Myophage Mu is a representative of contractile nanomachines with a simple tail baseplate. It has the capacity to infect a range of intestinal bacteria and has extensive applications in genetic engineering research. Using cryo-EM, we resolved the three-dimensional (3D) structures of the G(+) type phage Mu in both its extended state and urea-induced contracted state, the latter lacking the baseplate, at near-atomic resolutions. The structure of extended Mu can be divided into four distinct regions: the DNA-containing head, the connector complex, the tail, and the baseplate.

The baseplate was classified and reconstructed by using RELION software, generating a final resolution of 3.3 Å. The simple baseplate is comprised of eight protein components, including a hexameric tube initiator (gp43), a trimeric hub (gp44), a trimeric spike (gp45), six wedges (one BW1 gp46, two BW2 gp47, and one BW3 gp48), and six trimeric fibers (gp49 and gp50). The tube initiator protein gp43 is composed of two domains: a tube-like domain and a helix-rich domain, which are connected by a flexible loop. The tube-like domains from six copies of gp43 form a 24-stranded β-barrel hexamer, analogous to that of the tube gp40, which serves to initiate the assembly of the tail tube. It is noteworthy that the helix-rich domain comprises eight α-helixes, which extend downward and form extensive interactions with the baseplate wedges. The Mu spike protein gp45 is comprised of three domains: an oligosaccharide-binding (OB-fold) domain, a β-helical domain, and an apex domain, which may have the function of binding and penetrating the cell membrane. It is noteworthy that two additional spherical densities, which are presumed to be Fe and Ca ions, are present in the apex domain of the spike gp45, which is consistent with the reported X-ray crystal structure. As with myophages Milano, E217 (14), and Pam3 (13), the baseplate wedge of Mu is composed of six heterotetramers, each comprising one BW1 gp46, one BW3, and two conformers of BW2 (referred to as BW2-i and BW2-o). Moreover, the entire three-helical bundle is embedded between the helix-rich domains of two adjacent tube initiator gp43, thereby stabilizing the BWs into the baseplate. Based on our density map, we only built the atomic model for the N-terminus of protein gp49, which is anchored to the fiber docking loop (residues 133–155) of the BW3.

>[6x]MFEDALNAVNAVRDKTGGGRKTTGKGTFRNVPFLVIEEQKQAGGRRLVKREYPLRDTGGVNDLGKKLRSRTFSACILNSNAETARDEAGALMDALDAPGSGELVHPDFGTVDVMVDSWECRTKADELNYYAFTVTVYPSLQDTAPDAETDTSAAVPAQAVAVTGSLGDTLSSVWQTVKDGTAAATAVMEAVTGVIDDISDAVDNLGVTQTVSGLMGSLSAMKGSVTSLINQPAMLASSLMGALSGVSSLCDTRTAFSTWNRLAQRFERRHAATAGRQGTITTSYNSPVAEKNIATLNYVMLAAAQTYRAEAASQALTAALDFSRRMDNAARAPVLDAPSTTTGTASGASSTSATVTQGQLQLTAITPDGGFSQVSFSDSGTATPPVFESVSDIEKTTAMLGAALDSVILTASEQGFSTDSVQLTQLRLLVVADLEKRGLQLAGSESHHLPETLPAMVALYRFTGNSRNWQRLARRNGISNPLFVPGGVSIEVINE;>[6x]MSDISFNAIPSDVRVPLTYIEFDNSNAVSGTPAPRQRVLMFGQSGSKASAAPNVPVRIRSGSQASAAFGQGSMLALMADAFLNANRVAELWCIPQGNGTGNAAVGEISLSGTAGENGSLVTYIAGQRLAVSVAAGATGAALADLLVARIKGQPDLPVTAEVRADSGDDDTHADVVLSAKFTGALSAVDVRWNYYAGETTPYGIITAFKAASGKNGNPDISASIAGMGDLQYKYIVMPYTDEPNLNLLRTELQERWGPVNQADGFAVTVLSGTYGDISTFGVSRNDHLISCMGIAGAPEPSYLYAATLCAVASQALSIDPARPLQTLTLPGRMPPAVGDRFTWSERNALLFDGISTFNVNDGGEMQIERMITMYRTNKYGDSDPSYLNVNTIATLSYLRYSLRTRITQKFPNYKLASDGTRFATGQAVVTPSVIKTELLALFEEWENAGLVEDFDTFKEELYVARNKDDKDRLDVLCGPNLINQFRIFAAQVQFIL;>MAGNQRQGVAFIRVNGMELESMEGASFTPSGITREEVTGSRVYGWKGKPRAAKVECKIPGGGPIGLDEIIDWENITVEFQADTGETWMLANAWQADEPKNDGGEISLVLMAKQSKRIA[6x];>MTDLAIIWTNGRGDIAQDGIDMLTDDSLTTDVTISLFTDRRALDSDTLPDGSDDRRGWWGDSYRDRPIGSRLWLLSREKATPDTLERARGYAEEALEWLKTAGRVSAINVRAEQLHQGWLYLYIALTLPDGSVIPYEFKAAFNGV[6x];>MSNTVTLRADGRLFTGWTSVSVTRSIESVAGYFELGVNVPPGTDLSGLAPGKKFTLEIGGQIVCTGYIDSRRRQMTADSMKITVAGRDKTADLIDCAAVYSGGQWKNRTLEQIARDLCAPYGVTVRWELSDKESSAAFPGFTLDHSETVYEALVRASRARGVLMTSNAAGELVFSRAASTATDELVLGENLLTLDFEEDFRDRFSEYTVKGYARANGAEGDDIDAKSIVSRKGTATDSDVTRYRPMIIIADSKITAKDAQARALREQRRRLAKSITFEAEIDGWTRKDGQLWMPNLLVTIDASKYAIKTTELLVSKVTLILNDQDGLKTRVSLAPREGFLVPVESDRKNRKGGDSNGGIDALVEDYYRRHPEKTPPWKE[3x];>MAYSPPTLSSLIARTEQNIEQRLPGSWPQAREKTLSAIAYAQAGLAAGCHEHISWVGRQIIPSTADEDELLEHCRFWGVRRKQATAASGPLTVTTSAATTIPAGTRWQRADGVVYSLADTIVIDRAGTTEITVTALAAGEAGNTGENTLLTLITPVACVVSDAITVKGFSGGADIESAAELLSRLEYRVQYPPFGGNQFDYVRWAREVSGVTRAWCFPTWKGGGTVGVTFVMDNRSNIFPQPADVERVADYIAGHTDPITGLIVGQPDGVNVTVFAPKAKPVNPRIYISPKTAELKQAITNAINTMFFNEVMPGGALAPSRIIRAVAGVTGLDDFEVRFPTEIQRSENTELLTAGTIEWL[12x];>MERVNDSALNRLLTPLMRRVRLMLARAVVNVINDGRKVQNLQVGLLDDEESDEVERLQNYGHFSVPLPGAEALIACVGAQRDQGIAVVVEDRRYRPTNLEPGDAGIYHHEGHRIRLTKDGRCIITCKTVEVYADESMTVDTPRTTFTGDVEIQKGLGVKGKSQFDSNITAPDAIINGKSTDKHIHRGDSGGTTGPMQ[3x];>MAVTPWQTAFLQLLPSGLAWNKSPDSKLSALAQAISDVIATAADDARQMLRERFPSTSRWYLGEWESFLGLPDCTSENGTLSERQRAAANKMRMTGNLSRRFYEWLAAQYGFTVRLTDSTEGQWVTQVNIYGIKNYRNATVLDNVLTPLRVYESGALECLLEKYKPAHQIYKFVYHDGDN[6x];>[3x]MTGKRLKASVIIDLNGNLSRRSRQYSNQINALSRSGQSSLRALRMEVVRVSGAIDRMGSLSTRTFRMLSAGALGIAGVGYTANKLFIGAAAQREQQIIAMNSLYHGDKVRAQAMMAWAKQNAKDTTWGLSGVLDEIRSSKGFGMTDEQTKQFITMLQDQGAMHGWDLPTAQGASLQLKQMFARQQITAADANLLTGYGINVYQALADATGTDVKKIRDLGTKGKLGMKSILTVFRTLSEQSKGAQASAMNSWDGMFAQMEANLLEFRIKVANSGPFEEIKNEMRRVLNWHDMADKSGELDALAENIGQKFLTTFRTVKISAQELWRWLKPGKDALAWVDQNIVSLKKLAAVLVSVWLANKALRAGWAVAKPSWQVASYPFKTGRRMWRWMRNRKRGQAGLPVPDAMTSETLLQGIGIQRVFVINWPRGFGDYGSGGGRRVRSGGRMAPLLPRQPLLLSGPQPLALPAPRPVLALPPPGVPVTARPAPLPLPGKSGLLSRLAGSAAGQLVTGTVGKLADAGRAVGGWFSGIGNKLAGSAIGRVVTKGAGALGWMGKGAGRALSRLGGPVMGALQLAPVLMDEQASTHEKAGAIGSTAGAWLGGAVGSLAGPLGTVAGATLGSVAGEYLGGFVTDLYQKWTATDKEPQEQKVNAEASLRVELGEGLRLTSSRVTEDGMGLNIYAGDNYITGW;>[9x]MFYIDNDSGVTVMPPVSAQRSAIVRWFSEGDGNNVITWPGMDWFNIVQAELLNTLEEAGIQPDKTKLNQLALSIKAIMSNNALLIKNNLSEIKTAGASAQRTARENLDIYDASLNKKGLVQLTSATDSPSETLAATAKAVKIAMDNANARLAKDRNGADIPNKPLFIQNLGLQETVNRARNAVQKNGDTLSGGLTFENDSILAWIRNTDWAKIGFKNDADSDTDSYMWFETGDNGNEYFKWRSKQSTTTKDLMNLKWDALSVLVNAIVNGEVISKSANGLRIAYGNYGFFIRNDGSNTYFMLTNSGDNMGTYNGLRPLWINNATGAVSMGRGLNVSGDTLSDRFAINSSNGMWIQMRDNNAIFGKNIVNTDSAQALLRQNHADRKFMIGGLGNKQFGIYMINNSRTANGTDGQAYMDNNGNWLCGAQVIPGNYANFDSRYVRDVRLGTQSLTGGLSRDYKAPSGHVITGFHTNGDWEMQGGDDKVYIRPVQKNINGTWYNVASA>[4x]SHNMSLPQWCPPHSTLKRNPTTGEDVYCICKRPDYGELMVGCDGCDDWFHFTCLHIPEQFKDLVFSFYCPYCQAGITGKNKNGEGSLPKTLWKRKCRISDCYKPCLQ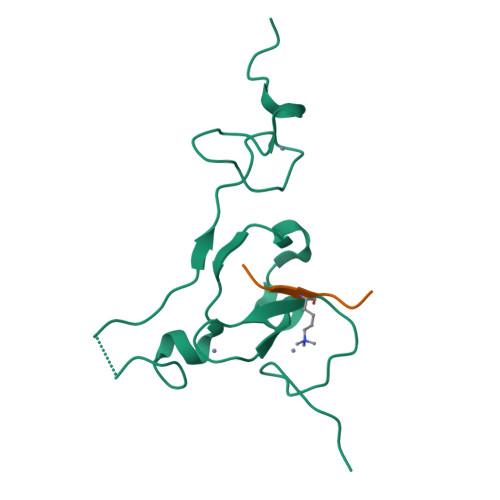DSKYCSEEHGREFVND;>[4x]ARTKQTA> HLSDMLQQLHSVNASKPSERGLVRQEEAEDPACIPIFWVSKWVDYSDKYGLGY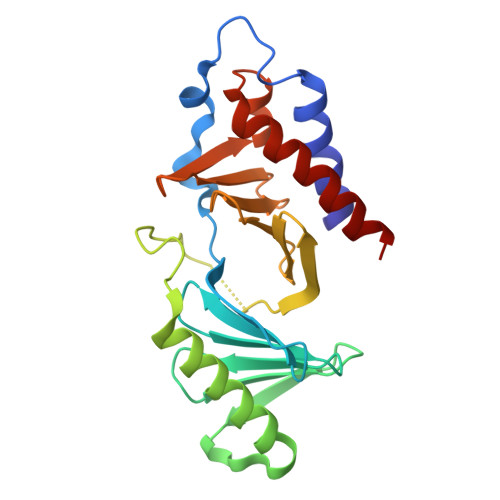QLCDNSVGVLFNDSTRLILYNDGDSLQYIERDGTESYLTVSSHPNSLMKKITLLKYFRNYMSEHLLKAGANITPREGDELARLPYLRTWFRTRSAIILHLSNGSVQINFFQDHTKLILCPLMAAVTYIDEKRDFRTYRLSLLEEYGCCKELASRLRYARTMVDKLLSS>[2x]GPLGSMSGTLVQRLKLILSGGNLRCSDGETACDPERPPTRCVFQVHGQDGSNDTFPL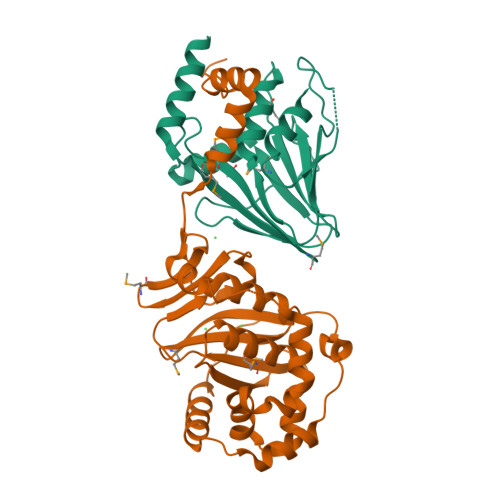EYVLRLMRSWAHVPCDPYVRVQNTGVSVLFQGFFFRPADAPLAAITAEHNNVILASTHSTGMSLSALDDIKRAGGVDTRPLRAMMSVSCFVRMPRVQLSFRFMGPDDASQTQRLLDRAELRQRS;>[2x]GPGSKTLTRAARDRYAPYFAYAAAQPSDEVTTVRGLSNPLIKTAPVTLPFDLGQAVADNCLSLSGMGYYLGLGGCCPTCAAAEPRLGRSDRAALVLAYVQQLNSIYEYRVFLASVAARDPSERALEEVLAHPELFFAYYVLRDGGLRDVRVLFFEDPDAQGALMMYVVFPEKSVHVHHRVLDRLLGACAGHRIVAHVWQTMFVLVVRKKGDGRPADDVPAVSASDIYCKMRDISFDGELLLEYKRLYAAFEDFRPPRP Here, we report the identification of human METTL13 as a dual MTase that targets both the N terminus and Lys55 of eEF1A through two distinct MTase domains, firmly establishing its function using a combination of in vitro and in vivo methods. METTL13 harbors two distinct predicted MTase domains that both belong to the 7BS superfamily. The N-terminal domain (here denoted MT13-N) belongs to a recently discovered enzyme family consisting of likely KMTs15 and the C-terminal domain (here denoted MT13-C) lacks close paralogs, but is distantly related to spermidine synthase (SpdS). During elongation, eEF1A performs the essential function of delivering aminoacyl-tRNA to the ribosome, in a process where the ribosome samples the available pool of ternary aminoacyl-tRNA–eEF1A-GTP complexes.

To obtain further insights into its molecular mechanism, we determined the crystal structure of its core MTase domain (residues 470–699) in complex with S-adenosylhomocysteine (AdoHcy), which is a byproduct of the methylation reaction, representing the demethylated form of AdoMet. Based on its sequence, MT13-C belongs to the family of Rossmann fold-like 7BS MTases, and, correspondingly, the determined structure of the MT13-C MTase domain reveals a classic 7BS structure, consisting of a twisted 7BS sheet surrounded by six α-helices, three on each side. Although the homocysteyl moiety of AdoHcy was not fully resolved by electron density, the MT13-C structure indeed revealed that residues in these motifs (Gly503 and Glu524 in METTL13) are involved in AdoHcy coordination, and show a similar positioning as in SpdS (in complex with MTA). Moreover, MT13-C and SpdS share a short DG-motif (Asp551-Gly552 in METTL13) localized after β-strand 3 and not generally found in other 7BS enzymes. The localization and orientation of the acidic aspartate residue in this motif allows hydrogen bonding to the primary amine of the adenosine moiety of AdoHcy and MTA, respectively. For SpdS, two aspartate residues (Asp173 and Asp176) in Post II have been shown to be important for both tetramethylenediamine (putrescine) substrate binding and efficient catalysis, and interestingly, MT13-C has an aspartate residue (Asp575) at the position corresponding to Asp173. Also, the other residues of motif Post II show a similar positioning between the two enzymes and MT13-C, in particular, also has an aspartate residue (Asp577) in spatial proximity to Asp176 in SpdS. To explore how MT13-C interacts with its peptide substrate, we modeled the 6-mer peptide (GKEKTH) corresponding to the N terminus of eEF1A onto the MT13-C structure by molecular docking. The highest-ranking docking model placed the substrate peptide in an evolutionary conserved groove with its N terminus oriented toward AdoHcy, i.e., an orientation very similar to that of putrescine in SpdS.

> MHHHHHHSSGRENLYFQGCCEHHKAMIAGLALLRNPELLLEIPLALLVVGLGGGSLPLFVHDHFPKSCIDAVEIDPSMLEVATQWFGFSQSDRMKVHIADGLDYIASLAGGGEARPCYDVIMFDVDSKDPTLGMSCPPPAFVEQSFLQKVKSILTPEGVFILNLVCRDLGLKDSVLAGLKAVFPLLYVRRIEGEVNEILFCQLHPEQKLATPELLETAQALERTLRKPGRGWDDTYVLSDMLKTVKIV>AYLLFYTEAKVTATVK[7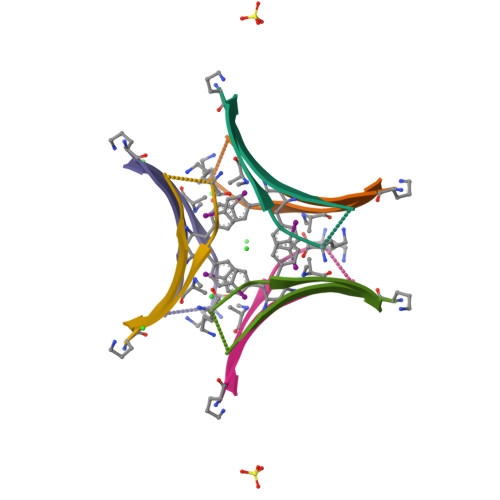x]> EPLYENSPEFTPYLETNLGQPTIQSFEQVGTKVNVTVEDERTLVRRNNTFLSLRDVFGKDLIYTLYYWSGKKTAKT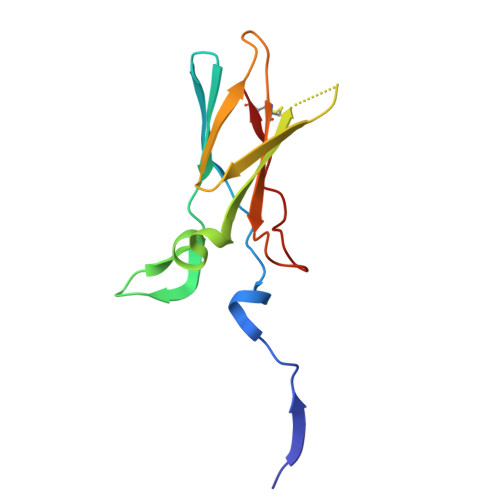NTNEFLIDVDKGENYCFSVQAVIPSRTVNRKSTDSPVECM>EKFLVIAGMNAIESEELLLKVGEEIKRLSEKFKEVEFVFKSSFDKANRSSIHSFRGHGLEYGVKALRKVKEEFGLKITTDIHESWQAEPVAEVADIIQIPAFLCRQTDLLLAAAKTGRAVNVKKGQFL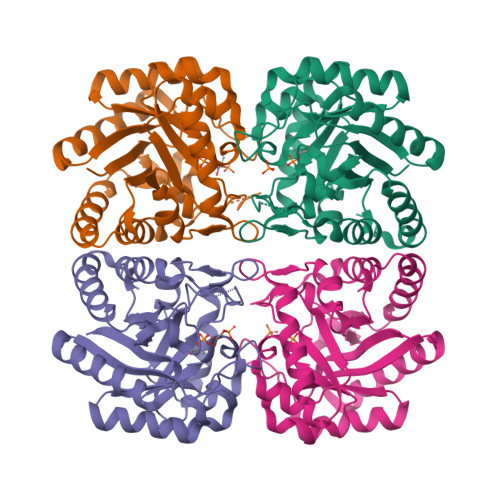APWDTKNVVEKLKFGGAKEIYLTERGTTFGYNNLVVDFRSLPIMKQWAKVIYDATHSVQLPGGLGDKSGGMREFIFPLIRAAVAVGCDGVFMETHPEPEKALSDASTQLPLSQLEGIIEAILEIREVASKYYETI[12x]> DLEELL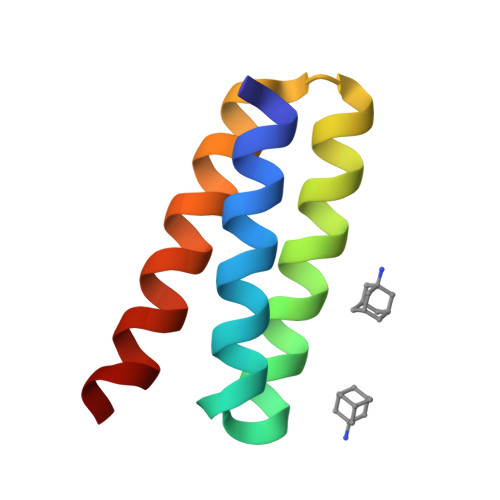QKIKEIVLKVMDIGDDETIKRAQKLLIKAELAVQKKDLKEVEKLLKEAEKVYKEVKEA>[2x]ATVGKVIKCKAAVAWEANKPLVIEEIEVDVPHANEIRIKIIATGVCHTDLYHLFEGKHKDGFPVVLGHEGAGIVESVGPGVTEFQPGEKVIP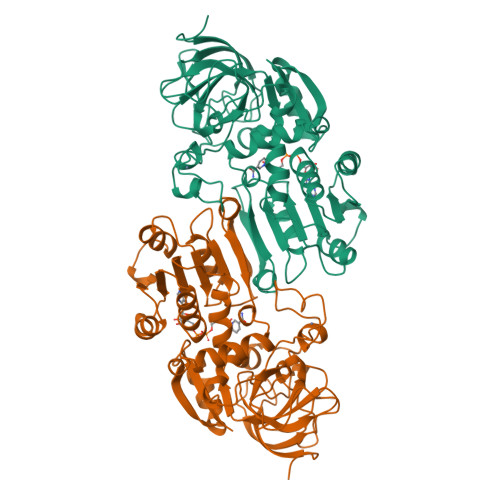LFISQCGECRFCQSPKTNQCVKGWANESPDVMSPKETRFTCKGRKVLQFLGTSTFSQYTVVNQIAVAKIDPSAPLDTVCLLGCGVSTGFGAAVNTAKVEPGSTCAVFGLGAVGLAAVMGCHSAGAKRIIAVDLNPDKFEKAKVFGATDFVNPNDHSEPISQVLSKMTNGGVDFSLECVGNVGVMRNALESCLKGWGVSVLVGWTDLHDVATRPIQLIAGRTWKGSMFGGFKGKDGVPKMVKAYLDKKVKLDEFITHRMPLESVNDAIDLMKHGKCIRTVLSL N-ALPHA-(2-NAPHTHYLSULFONYL)-N(3-AMIDINO-L-PHENYLALANINYL)-4-ACETYL-PIPERAZINE 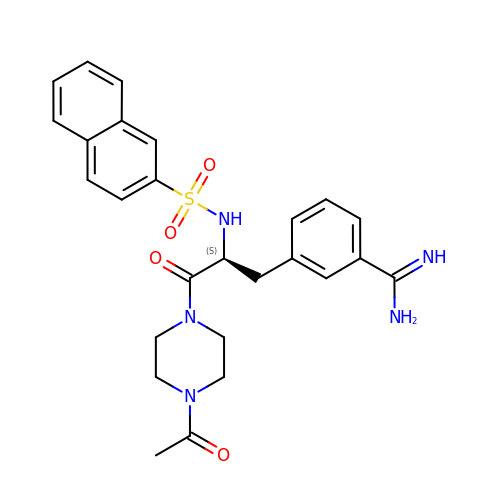| C26 H29 N5 O4 S | ZUWBXGHMVKDMQO-DEOSSOPVSA-N>GMALQLSREQGITARGSAEIVAEFFSFGINSILYQRGIYPSETFTRVQKYGLTLLVTTDLELIKYLNNVVEQLKDWLYKSSVQKLVVVISNIESGEVLERWQFDIESDKTAKDDSAPREKSQKAIQDEIRSVIRQITATVTFLPLLEVSCSFDLLIYTDKDLVVPEKWEESGPQFITNSEEVRLRSFTTTIHKVNSMVAYKIPVND[12x]

A cellular surveillance system called the spindle checkpoint ensures that accurate chromosome segregation occurs by inhibiting the activity of the anaphase-promoting complex or cyclosome (APC/C) until all sister chromatids have achieved proper attachment to the mitotic spindle. The spindle checkpoint protein Mad2 binds to Cdc20, an activator of APC/C, and inhibits the complex. The Mad2 protein can adopt either an open or closed conformation. The conformational switch in Mad2 is critical for Cdc20 binding and APC/C inhibition, and is regulated by the protein Mad1.

C79 and C106 of Mad2 are located in close proximity and tend to form an intramolecular disulfide bond, causing conformational heterogeneity. To facilitate crystallization, we created a Mad2L13A,C79S,C106S triple mutant, which retained its abilities to bind to Cdc20 and inhibit APC/C in vitro (see below). However, we obtained crystals of Mad2L13A that diffracted X-rays to a minimum Bragg spacing of 1.95 Å and determined its structure using molecular replacement. The two monomers mainly interact through the C-terminal halves of their αC helices. The dimerization interface of Mad2L13A is symmetric and consists of residues from the C-terminal half of αC, R184 from β8′, and Q34 at the C-terminal end of αA. These residues form hydrophobic interactions and extensive networks of water-mediated hydrogen bonds. Bridged by two tightly bound water molecules, R133 from one monomer forms a network of hydrogen bonds with both the backbone and side-chain carbonyl groups of Q34 and the backbone carbonyl of T136 from the neighboring monomer. In unliganded C-Mad2, F141 points outward and engages in numerous interactions at the dimerization interface. Thus, R184 of β8′ indirectly contributes to Mad2 dimerization by forming an intramolecular hydrogen bond with the side chain of Q134, explaining the inability of O-Mad2 to form symmetric dimers. Mad2L13A, which predominantly exists as the symmetric C–C Mad2 dimer, is functional in cells and is active in APC/CCdc20 inhibition in vitro.[(2~{R},5~{S})-1-[(2~{R},3~{S},4~{R},5~{R})-5-(6-aminopurin-9-yl)-3,4-bis(oxidanyl)oxolan-2-yl]-5-azaniumyl-6-oxidanyl-6-oxidanylidene-hexan-2-yl]-(phenylmethyl)azanium 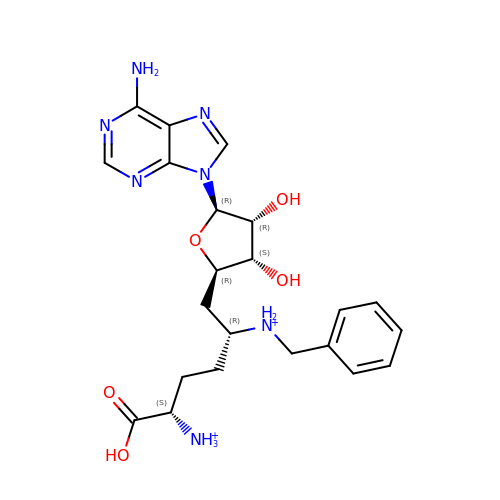| C22 H31 N7 O5 | FIOIMCLLFNYJFV-ZGTZEGHKSA-P>[2x]AYECGKQGGGALCPNNKCCSRYGYCGFGPAYCGTGCQSGGCCPGKRCGDQANGETCPNNLCCSEDGYCGFGSEY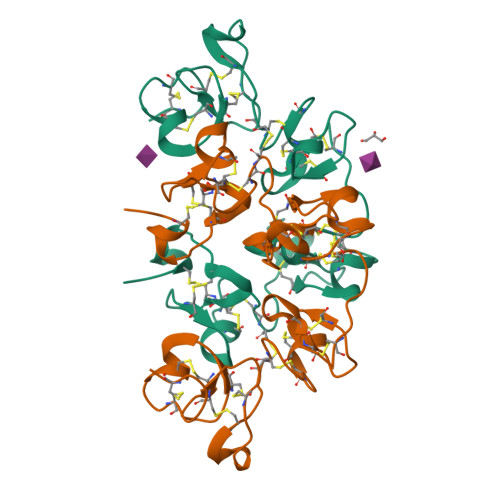CGAGCQGGPCRADKLCGTLAGGQLCPDNLCCSQWGFCGLGVEFCGDGCQSGACCSMRCGRQADGAKCTNNYCCGASGYCGLGGDYCGAGCQSGPCT>[4x]MEGTGVVAVYGNGAITEAKKSPFSVKVGLAQMLRGGVIMDVVNAEQARIAEEAGACAVMALERVPADIRAQGGVARMSDPQMIK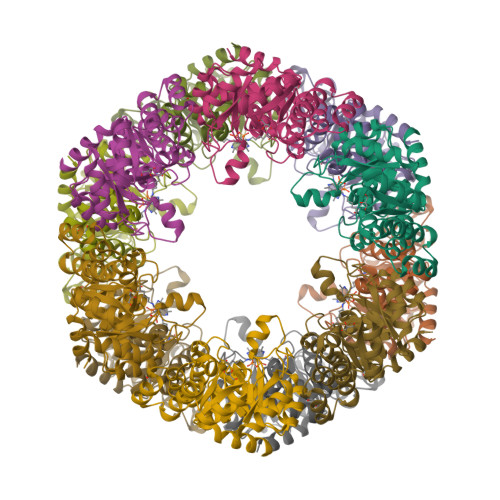EIKQAVTIPVMAKARIGHFVEAQILEAIGIDYIDESEVLTLADEDHHINKHNFRIPFVCGCRNLGEALRRIREGAAMIRTKGEAGTGNIIEAVRHVRSVNGDIRVLRNMDDDEVFTFAKKLAAPYDLVMQTKQLGRLPVVQFAAGGVATPADAALMMQLGCDGVFVGSGIFKSGDPARRARAIVQAVTHYSDPEMLVEVSCGLGEAMVGINLNDEKVERFANRSEEHHHHHH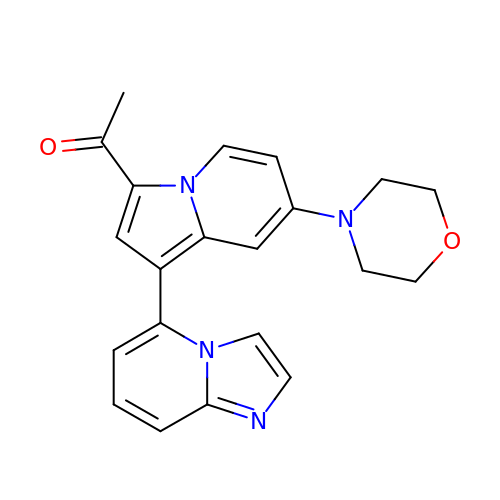1-[1-(imidazo[1,2-a]pyridin-5-yl)-7-(morpholin-4-yl)indolizin-3-yl]ethanone | C21 H20 N4 O2 | LBUBPCSKFDKKFO-UHFFFAOYSA-N>[5x]TTQPALLRLSDHLLANYKKGVRPVRDWRKPTTVSIDVIMYAILNVDEKNQVLTTYIWYRQYWTDEFLQWTPEDFDNVTKLSIPTDSIWVPDILINEFVDVGKSPNIPYVYVHHRGEVQNYKPLQLVTACSLDIYNFPFDVQNCSLTFTSWLHTIQDINITLWRSPEEVRSDKSIFINQGEWELLEVFPQFKEFSIDISNSY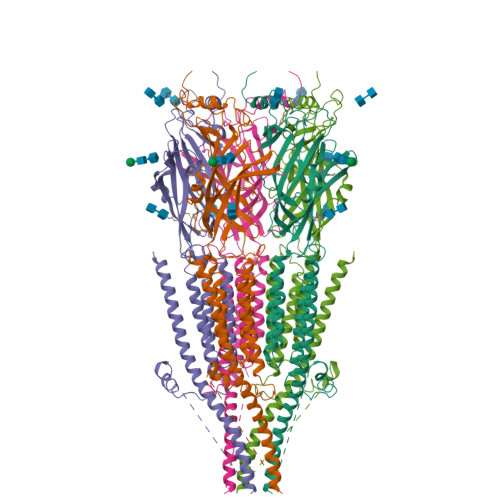AEMKFYVIIRRRPLFYAVSLLLPSIFLMVVDIVGFCLPPDSGERVSFKITLLLGYSVFLIIVSDTLPATAIGTPLIGVYFVVCMALLVISLAETIFIVRLVHKQDLQRPVPDWLRHLVLDRIAWILCLGEQPMAHRPPATFQANKTDDCSAMGNHCSHVGGPQDLEKTPRGRGSPLPPPREASLAVRGLLQELSSIRHFLEKRDEMREVARDWLRVGYVLDRLLFRIYLLAVLAYSITLVTLWSIWHYS>[6x]MQTKKNEIWVGIFLLAALLAALFVCLKAANVTSIRTEPTYTLYATFDNIGGLKARSPVSIGGVVVGR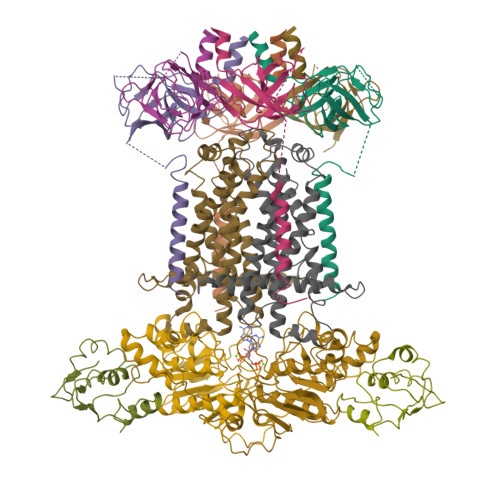VADITLDPKTYLPRVTLEIEQRYNHIPDTSSLSIRTSGLLGEQYLALNVGFEDPELGTAILKDGDTIQDTKSAMVLEDLIGQFLYGSKGDDNKNSGDAPAAAPGNNETTEPVGTTK;>[2x]MSESLSWMQTGDTLALSGELDQDVLLPLWEMREEAVKGITCIDLSRVSRVDTGGLALLLHLIDLAKKQGNNVTLQGVNDKVYTLAKLYNLPADVLPRHHHHHHHH;>MLLNALASLGHKGIKTLRTFGRAGLMLFNALVGKPEFRKHAPLLVRQLYNVGVLSMLIIVVSGVFIGMVLGLQGYLVLTTYSAETSLGMLVALSLLRELGPVVAALLFAGRAGSALTAEIGLMRATEQLSSMEMMAVDPLRRVISPRFWAGVISLPLLTVIFVAVGIWGGSLVGVSWKGIDSGFFWSAMQNAVDWRMDLVNCLIKSVVFAITVTWISLFNGYDAIPTSAGISRATTRTVVHSSLAVLGLDFVLTALMFGN[2x];>MEQSVANLVDMRDVSFTRGNRCIFDNISLTVPRGKITAIMGPSGIGKTTLLRLIGGQIAPDHGEILFDGENIPAMSRSRLYTVRKRMSMLFQSGALFTDMNVFDNVAYPLREHTQLPAPLLHSTVMMKLEAVGLRGAAKLMPSELSGGMARRAALARAIALEPDLIMFDEPFVGQDPITMGVLVKLISELNSALGVTCVVVSHDVPEVLSIADHAWILADKKIVAHGSAQALQANPDPRVRQFLDGIADGPVPFRYPAGDYHADLLPGS[2x]>[2x]ALYQLEKEPIVGAETFYVDGAANRETKLGKAGY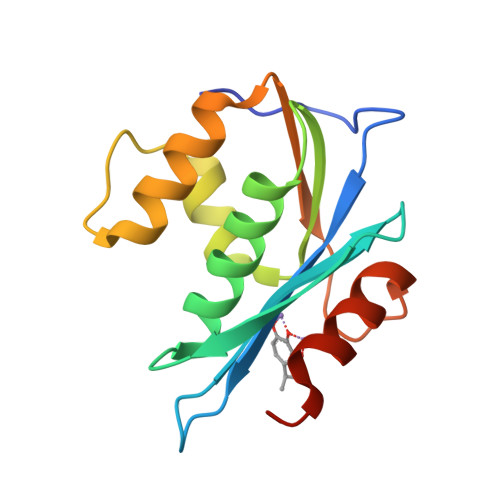VTNKGRQKVVPLTNTTNQKTELQAIYLALQDSGLEVNIVTDSQYALGIIQAQPDKSESELVNQIIEQLIKKEKVYLAWVPAHKGIGGNEQVDKLVSAGIRKIL>[2x]MYPGSGNYSYNNRPSMPPPGFNGDGQGYRQEYGNQYGGGYQQQQYQDQYQGENRGQYQGQYQDQPEYGRPPSGMVRPPSSIQQGNGQQFQYSQMTGRRKALLIGINYIGSKNALRGCINDAHNIFNYLTTYCGYRPEDIVMLTDDQREMVKIPLKENIIRAMQWLVKDAQPNDA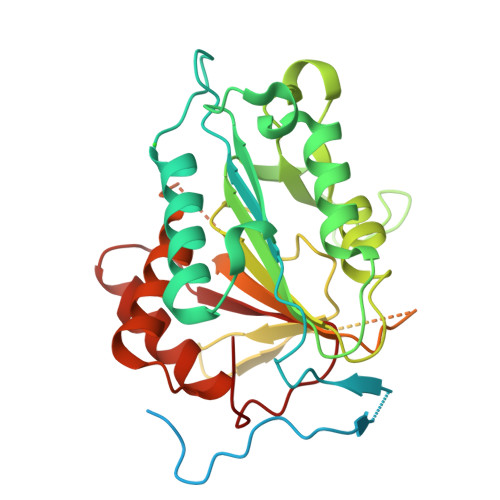LFFHYSGHGGQTKDLDGDEEDGMDDVIYPVDFESVGPLIDDTMHDIMVKSLPQGARLTALFDSCHSGTVLDLPYTYSTKGVIKEPNMWKDVGSDGIQAAMAYATGNRSALFSSIGNMVSSVTKKQNVDRERVRQIKFSPADVIMLSGSKDNQTSADTFADGQNIGAMSHAFISVMTRQPQQSYLSLLQNLRNELAGKYSQKPQLSASHPIDVNLQFIM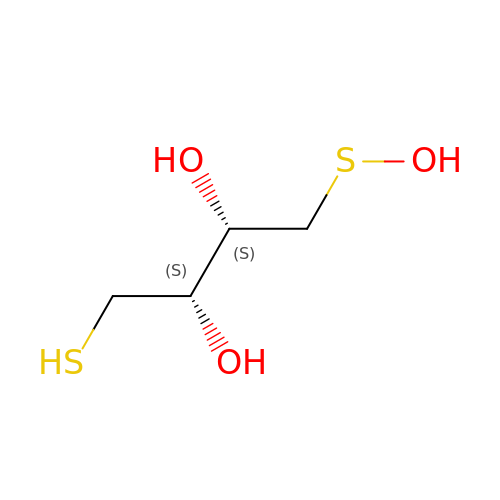1-HYDROXYSULFANYL-4-MERCAPTO-BUTANE-2,3-DIOL | C4 H10 O3 S2 | MFLGZMZEMVZQCC-QWWZWVQMSA-N It comprises a predicted β-barrel protein of the TBDR (TonB-dependent receptor) family, NanO (neuraminate outer membrane permease), adjacent to a smaller protein, NanU (extracellular neuraminate uptake protein) that has homology with the SusD family of proteins. In the present study, we present genetic, biochemical and structural data that elucidates the function of NanU as a high-affinity sialic acid-binding protein that works in concert with its cognate TBDR, NanO, in sialic acid transport. Specifically, we have established NanU as a novel member of the SusD family of proteins that binds sialic acid with a high affinity (Kd of ~400 nM). Therefore NanU, together with its partner porin NanO, forms part of an integrated sialic acid-uptake system present in several Bacteroidetes species which we suggest as the first sialic acid-specific PUL.

To characterize further the NanU protein, we determined the crystal structure of BF-NanU to a resolution of 1.6 Å. The crystal asymmetric unit shows clearly a monomeric form for the protein in agreement with our gel-filtration data, and an overall predominantly α-helical structure, reminiscent of several other members of the SusD family. We also report the structure of NanU at 1.6 Å and reveal that despite low sequence similarity with other SusD proteins (~20% at the amino acid level), there is a strongly conserved structural homology based mainly on the presence of a series of four α-helix-rich TPR units that define the scaffold for the structure of these proteins. With the exception of an extended β-ribbon and turn (Met344–Cys363) in BF-NanU and two small two-stranded anti-parallel β-sheets in SusD (Cys94–Trp96 and Ile323–Ala325 and Lys172–Phe175 and Val185–Lys188), the majority of structural differences lie within the loop regions. The α2 helix defines a motif pivoted around amino acid 50/51 (extending from Glu33 to Gly58) that is well conserved between the putative NanU proteins (residues highlighted in grey text), but not with non-sialic acid-related Sus proteins, namely SusD and BT1043 from B. thetaiotaomicron, both which are involved in oligosaccharide rather than monosaccharide binding. A second structural loop in SusD, seen to move upon substrate binding (residues 292–297), and thus provide a critical tyrosine-mediated contact, is present in BF-NanU (residues 276–280), but there are no structurally equivalent residues to the tyrosine and tryptophan residues that co-ordinate ligand in the SusD co-crystals. At present, we can only speculate as to the binding site for sialic acid, as we have tried repeatedly to produce ligand-bound crystals using various ligands with no success to date, but it seems possible that the observed differences in structure and amino acid composition may define the binding specificity of BF-NanU for monosaccharide derivatives, such as sialic acid, over the starch or oligomeric sugars observed in SusD family protein structures to date.

> MLAGLSLLLFSRCDALDIDPTSSIADSNYWKTEAQFSTFNVGLHALLRECSFNFFLLGEPRADIYGDVPFGGEATQGMERLPFNTINKENTGISNFAGMYKVINQINLMIAKTKETTVLSEAGKNYYLGEAYGMRAYLYFHLLRSWGDVILYLDYTNGASLDLSNLSKAASPAEEVMKQIKEDITASEKGFGSDYSFKYGRYYWSMAATQMLKGEVYLWSGRQMGGGTADYTTAKTALQSIVSNANVSLQDDFSKVFAYNNKDNSEIIFSIRNAKDEYNMWDDRFRQNLVPQQAYMTSTYCNKEGVSFKDLPEGQLNGLIRLQIRYDLYNKAFRDGDTRKDASMTAVYQKQQDGTVKYIAPFCNKYQGVLLDGASQRSFLNDYPIYRYADCLLLLAEAKALLGEDPTAEINQVRERAYGKEFFEANKATLAYPNDKGDFYTDNKYMSGDEDPLEAILKERMREFMFEGKRWYDLRLLGADYVTKRTSAVATRLLWPINESVLTDNPALKQTPGYQNEHHHHHH>KFGELREISGNQYVNEVTNAEEDVWVIIHLYRSSIPMCLLVNQHLSLLARKFPETKFVKAIVNSCIQHYHDNCLPTIFV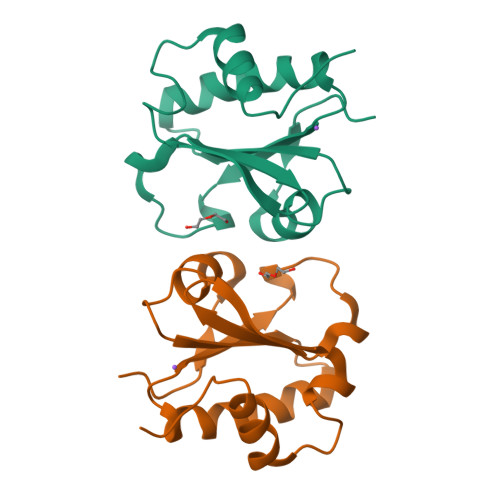YKNGQIEAKFIGIIECGGINLKLEELEWKLAEVGAIQTD[2x]>MPLPSPNLDDRRFQQFVDDAKRYIQQRAPEWTDHNVSDPGVTLVETVAHMADQIVYRLNRVPDKNHLAFLDLVGITLFPPSAARTDVTFWLSAPQEDAILVPVGTEVATLRTERDEAVVFATEQDLRIVPCTMGRLVTQVSGEAVSDRTTDLAESKDVLCFAEAPNPGDCMLIGLSAAVPDCALALELDSRVDGVGVDPRQPPLVWEAWTEDGWQSCEVDRDGTGGLNRPGDVVLHIPGGHVLSRNGGHEAGWIRCRVTEPLSGQPFYTTSPTIRSAEAYTIGGTTGSIHAETVLDEPLGESTGLPGQRLRLEHAPVVAGEPSVLLQTAADDGWQDWQVVPHFSGSHPDDHHITVDATTGEIAFGPAVREADGTLRQYGAVPPKGAVIRARRYRTGGGRAGNVARGAVQVLRTSIPYVSEVVNREAALGGVDGETIEEAKLRAPITLRAQERAVTLRDYEELARRAAPETARITCLEGAENEYGAHAVRVLVVPQAVPDPGGRLRFEQLVPGDALLNRITRHLDERRLIGTRLAVGPPYYQGVTVVATVHAFRDVDADRVRRQTHDALYRHLDPLTGGSDGKGWPFGRPVQTGELFAVLQRVPGVELVDEVVLHPADPLTGKRGDPTNRIDLDAPALVFSYDHRVRVIGDSA[12x];>MPSYLSPGVYVEEVASGSRPIEGVGTSVAAFVGLAPTGPLNEPTLVTNWTQYVAAFGDFTGGYYLAHSVYGFFNNGGSAAYVVRVGGSAEDAAADGSVNGAAAPAAVTGSTAKALPAAEPKQLGTFAVTATAAGQSGPLTVEVADPEGEGPAERFKLIVKDGDKPVETFDVSAKKGNRSYVVTQVKERSKLITVTEAAPSAQLVRPENQSLTLPAPPSAAPAVPAGQAESAHPGPAQYLGDSSDRTGFGGLEAIDEISMVAVPDLMAAYQRGAIDLEAVKAVQLGLIAHCELMGDRVAIIDPPPNQNARQIRVWRQETAGYDSKYAALYYPWIKSFDPATGQSRLVPPSGHVAGIWARNDSERGVHKAPANEVVRGAVDLELQITRGEQDLLNPIGVNCIRSFPGRGIRVWGARTLSSDPAWRYLNIRRYFNYLEESILIGTQWVVFEPNDHNLWARIRRNVSAFLVNEWRNGALFGQSPDQAYYVKCDEETNPPESVDLGRVVCEIGIAPVKPAEFVIFRLAQFSSGGGELDE[18x];>[6x]MKPASQRGSVDGLGSSLPIASMLPAVFADDDLALRFVAGLDDVLAPILNVLDCLDTYFDPALTPADFAQWLGTWVGAETDGTEAEPMLRAAVAAAARLHRVRGTLQGLSETVRLAFGVAPEITESGGATWNARPLGPFPGRPRPQLHVALRLPEPRPVDVHRLDALVAAARPAHMPYTVEVTASERTPER;>[6x]MAKSSKGAGKSLVRANLAIHEPPTGKSTSPGGLIKRFPFEFNPAQLSISQRSQWKATPTAAVRKAAKPQFMGAEPREMTLEIFLDSSMKPGGNTVMKKVESLLICCEVTAKSLAAKQPSPPWVIFEWGSFSTARFNAYVASIETQYTLFGTAGVPIRATCQMGLVEIPGPTPNQNPTSGALTAQRVHRVVAGDSLQSLAWSEYGSANAWRVIAEANGIDDPSHLPTGTELILPATEEVPH;>[6x]MAEQFVGSGWSFPLRIGPTGGIALVSGEQEVEEAMRLILATAPGERPMRPEFGCAIHDLVFAPVNEQTAGRIQHEVYVTLDRWEPRIEVHDVDVTTGEEQNVLFIDVRYSIRGTNNPRSLVFPFYVIPSHDEPDLPDAPAGLPGSPESDR;>[6x]MTRKDPGSSIWFSLAIDGESLGYFNGCEGLSTQVEVEQRQEGGNNGFVWQLPTRVTYSNIRLTRPLTPDTAKVAKWISSVQTGIQRPTAQISALRADGSLVARWGLIDVLPVSWQGPSLDPGSASVANEVLEIAHHGFTD;>MSLPKPEDVLVAPNFGIQIDGVMVEYLNSVSNLQIEQDVIRYQQNQGTTGRNNVTLMPGVAKDGSVQVERGMSQSSVFTQWINDSMAGRMATARKNATIIVMDYEDNPVKRWNLRNAWCSKVVAGTLKAGDTNALTETITIVFEELVVE[6x]

Bacterial contractile injection systems (CIS) are phage tail-like macromolecular complexes that mediate cell-cell interactions by injecting effector proteins into target cells. Using Streptomyces coelicolor as a model organism, we and others previously demonstrated that S. coelicolor CIS (CISSc) mediate a form of regulated cell death, which influences the onset of sporulation and secondary metabolite production in response to exogenous stress and unknown cellular signals (Casu et al., 2023; Vladimirov et al., 2023). The purified assemblies were subjected to single-particle cryo-electron microscopy (cryoEM) for structure determination, yielding the first high-resolution model of the CISSc in its extended conformation, which also presents the first example of a CIS IId subtype. Our model shows that extended CISSc particles share the conserved eCIS architecture, including the three core modules: cap, sheath tube, and baseplate.

The baseplate module comprises a heteromeric assembly of the proteins Cis1b/7/8/9/11/12. The symmetry transition from the inner tube (Cis1a, C6) to the VgrG-like spike (Cis8, C3) is adapted by two layers of the tube initiators Cis1b and Cis7. The first layer of the sheath (Cis2) is bound to the conserved gp25-like protein Cis9, which connects to the baseplate ‘wedges’ composed of Cis11 and Cis12. Importantly, the CISSc ‘wedges’ consist of two copies of Cis11 and one copy of Cis12, resembling the baseplate of Pyocin R2(27). This is in contrast to other previously reported eCIS, whose baseplate wedge comprises only one Cis11/12 component (AlgoCIS, AFP, PVC) and a Cis11 extension forming a cage around the spike (AlgoCIS; Xu et al., 2022; Jiang et al., 2019; Desfosses et al., 2019). (f) Ribbon diagrams showing a single baseplate wedge subunit, which is composed of two copies of Cis11 and one copy of Cis12. Furthermore, we did not detect any structural components that resemble tail fiber proteins. Interestingly, this analysis identified the baseplate component Cis11 as a significant hit and possible interaction partner of CisA. Importantly, such a protein-protein interaction would be consistent with our cryoEM structure, which shows a peripheral surface-exposed position of Cis11 in the baseplate complex of extended CISSc. The resulting maps of the baseplate and the cap reached resolutions of 3.5 and 3.4 Å, respectively.> MPFPFGKSHKSPADIVKNLKESMAVLEKQDISDKKAEKATEEVSKNLVAMKEILYGTNEKEPQTEAVAQLAQELYNSGLLSTLVADLQLIDFEGKKDVAQIFNNILRRQIGTRTPTVEYICTQQNILFMLLKGYESPEIALNCGIMLRECIRHEPLAKIILWSEQFYDFFRYVEMSTFDIASDAFATFKDLLTRHKLLSAEFLEQHYDRFFSEYEKLLHSENYVTKRQSLKLLGELLLDRHNFTIMTKYISKPENLKLMMNLLRDKSRNIQFEAFHVFKVFVANPNKTQPILDILLKNQAKLIEFLSKFQNDRTEDEQFNDEKTYLVKQIRDLKRP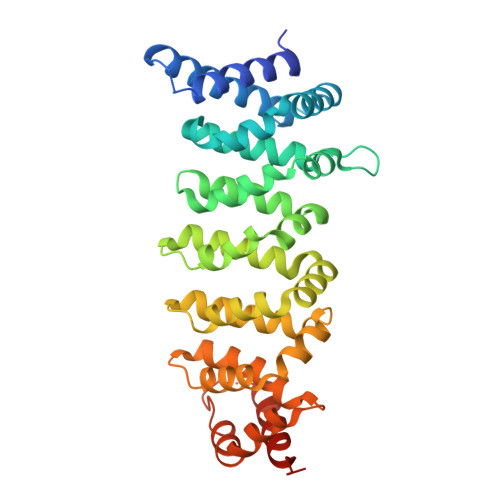AQQEA>[2x]MREESWEDHDTIQLTAQRKYLAEVQALETLLTRELSVFLTEPGSKKTNIINRITGKTYALPSTELLRLYEHLEQCRKQGALMYFLERQGTYSGLMLDYDLKLNTNAVPPLEPPALSRLCHRIFVHIKNSSVLPEGSHKIHFFFTLKPEVVQGKYGFHVLIPGLKLAASTKKS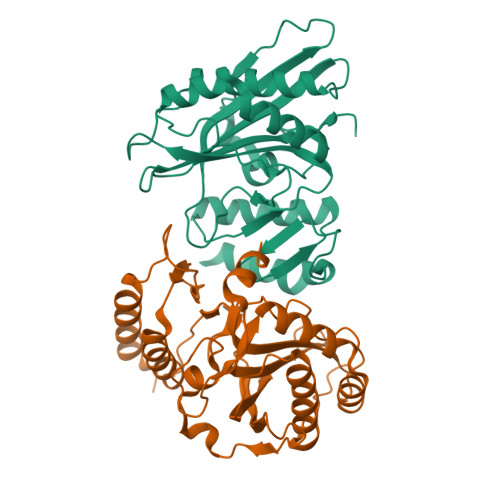IIGSLQHDATVQKILHEQGVTNPESCLDPHSASVPSLLYGSSKLNHKPYQLKTGFELVFDSSDPDYIPIHQIKNLESYNLVSELSLTNEQGSLVRPVYCAADIAAEKEEEIP In conclusion, we identified and characterized Paenibacillus spp. NagB1 and NagB2 proteins as SBPs for chitin oligosaccharides. Binding experiments of the recombinant NagB1 and NagB2 to several oligosaccharides using differential scanning fluorimetry and surface plasmon resonance confirmed that both proteins are SBPs of (GlcNAc)2 and (GlcNAc)3. SBPs, a component of ABC transporters, are responsible for trapping ligands that are imported through a specific pathway formed by two TMDs, and mainly define the specificity and affinity of transporters (Berntsson et al., 2010, ter Beek et al., 2014). The structures of NagB1 and NagB2 were classified as subcluster D-I and contained two α/β domains connected by a hinge region consisting of three strands, with the substrate-binding pocket located between the two domains.

The crystal structures of NagB2 in ligand-free or complex forms with (GlcNAc)2 (NagB2/(GlcNAc)2) and (GlcNAc)3 (NagB2/(GlcNAc)3) were determined at 1.2 to 1.8 Å resolution. There were two polypeptide chains in the asymmetric unit of the crystal of the ligand-free form (chain A, Asp47–Leu452 and chain B, Val49–Gly450), whereas there was only one polypeptide chain in the ligand-bound form. In contrast, in the asymmetric unit of the ligand-free crystal of NagB2, the two polypeptide chains showed two different opening structures. The inter-domain rotation angle between the two chains was 27.1° and belonged to an open form (chain A) and a semi-closed form (chain B). When (GlcNAc)2 was bound, this angle changed to 56.8° between the closed and open forms and 30.2° between the closed and semi-closed forms. When (GlcNAc)3 was bound, the angles were 58.6° between the closed and open forms and 32.1° between the closed and semi-closed forms. Upon binding to the ligand, SBP undergoes a conformational change from an open conformation to a closed conformation. This change is known as the “Venus flytrap” mechanism (Berntsson et al., 2010, Mao et al., 1982, Tirado-Lee et al., 2011, Vyas et al., 1988). The structure of NagB2 also changed significantly upon ligand binding, and the rotation angle was comparable to that of previously known structures.

>[2x]MGCGGTADKNPAGNNGDSAKPAETKSGDSVSLTLRHINVRDTAKNTLALLEKVVKKTEAEVPGATFKLDGVEDTVNRDVKLKAEMAAGKPPQIFNLFGGADTQNYAKAGHLLPLNDILKELGLEDKFFELREFTVDGKIYGLPEAGFVEGFYYNTKLFADAGITSAPKTWDEFTKALEALKAKNITPIALGGGSGDGWAINMLANSLFVATAGPEAQEGFAKGTTKWTDPAVLDGFKRLKDLKDKGYIDPNVLGLKYSEGQAKFYTGQAAMLFDGSWATSAILDKDKSTVKDNVGYFRFPNIGGKGDNLINGGWSNGYGFSSHLNDAEKKAVKAFIKNFYTLEIQGEALGRDNRVPSMKGVPTPAEAAPLTKAIGEAQASAKAAFPAFDALVQPKVKVTLEQSVQELLGGQLTPEKLVEKMQKVQDEANAGKLEHHHHHH1~{H}-1,2,3,4-tetrazol-5-ylmethyldiazane | C2 H6 N6 | 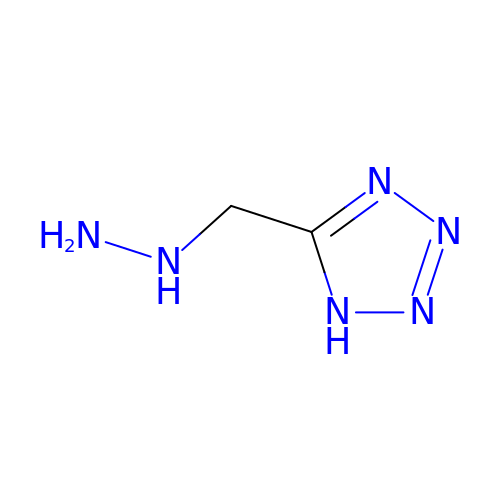LKTRPEVOGNHGTR-UHFFFAOYSA-N>GSHMPVPSFGEAMAYFAMVKRYL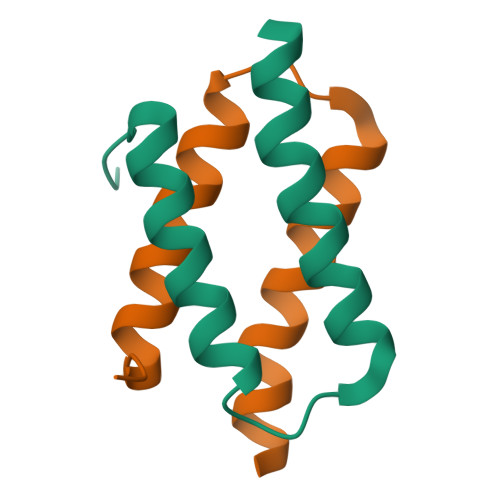TSFPIDDRVQSHILHLEHDLVHVTRKNHARQAGVRGLGHQS[4x]> LSYPNATESVYGLTRYSTNDEAIAGVNNESSITPAKFTVALNNVFETRVSTESSNGVIKISSLPQALAGADDTTAMTPLKTQQLAVKLIAQIAPSKNAATESEQGVIQLATVAQARQGTLREGYAISPYTFMNSTATEEYKGVIKLGTQSEVNSNNASVAVTGATLNGRGSTTSMRGVVKLTTTAGSQSGGDASSALAWNADVIHQRGGQTINGTLRINNTLTIASGGANITGTVNM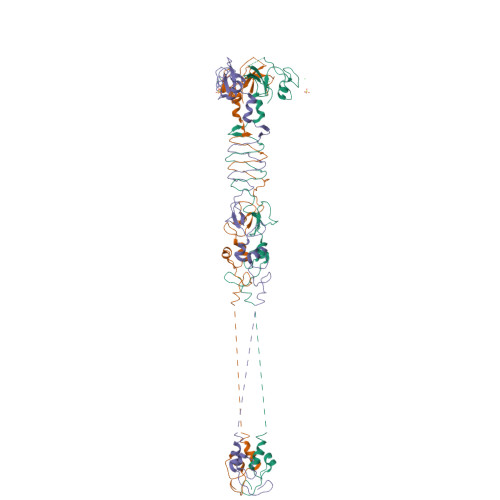TGGYIQGKRVVTQNEIDRTIPVGAIMMWAADSLPSDAWRFCHGGTVSASDCPLYASRIGTRYGGSSSNPGLPDMRSLNYIIKVKE> GAGCAGACCTGA;> CGGAACTCA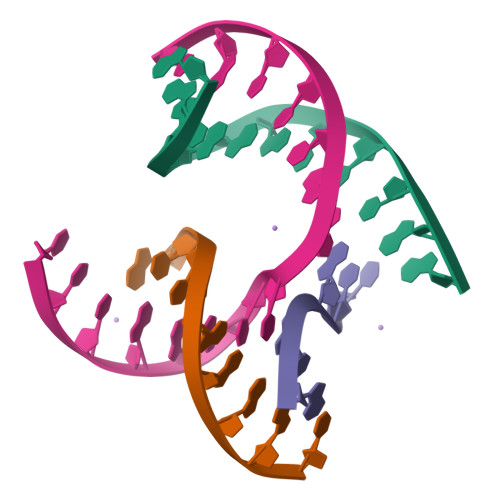;> TCACCG;> TCTGAGTTGGTCTGC> SELDPKGQHVCVASSPSAELQCCAGWRQKDQECTIPICEGPDACQKDEVCVKPGLCRCKPGFFGAHCSSRCPGQYWGPDCRESCPCHPHGQCEPATGACQCQADRWGARCEFPCACGPHGRCDPATGVCHCEPGWWSSTCRRPCQCNTAAARCEQATGACVCKPGWWGRRCSFRCNCHGSPCEQDSGRCACRPGWWGPECQQSRHHHHHH

SCARF1 (scavenger receptor class F member 1, SREC-1 or SR-F1) is a type I transmembrane protein that recognizes multiple endogenous and exogenous ligands such as modified low-density lipoproteins (LDLs) and is important for maintaining homeostasis and immunity. SCARF1 (MW, 86 kD) is a type I transmembrane protein that has a short signal peptide followed by a long extracellular region, a transmembrane helix, and a large cytoplasmic portion (Adachi et al., 1997). Its ectodomain has three glycosylation sites and contains multiple EGF-like domains, which usually has a two-stranded β-sheet followed by a loop region and three conserved disulfide bonds. Here, we solve the crystal structures of the N-terminal fragments of human SCARF1, which show that SCARF1 forms homodimers and its epidermal growth factor (EGF)-like domains adopt a long-curved conformation.

Among them, two fragments (f1, 20–132aa and f2, 20–221aa) were crystallized and the crystals diffracted to 2.2 Å and 2.6 Å, respectively. The structure of f2 fragment was solved by molecular replacement using the structure of f1 fragment combined with the EGF-like fragments predicted by AlphaFold as phasing models and refined to 2.6 Å resolution. The crystal belongs to space group P4122 with one molecule per asymmetric unit. In the f2 crystal structure, the N-terminal region of SCARF1 (residue 20–56aa) and the C-terminal region (210–221aa) are largely missing, suggesting these regions are quite flexible, consistent with low electron density of the N-terminal end of the f1 crystal. Rest of the f2 fragment adopts a long-curved conformation with multiple EGF-like domains arranged in tandem. Interestingly, in the crystal of f2 fragment, although an asymmetric unit has only one molecule, the dimer related by the crystallographic twofold symmetry can be well superimposed with the dimer found in the asymmetric unit of f1 crystals, suggesting that dimerization occurs in a similar fashion for the two fragments in different crystal forms. At the dimeric interfaces of f1 and f2 fragments, hydrogen bonds are formed between S88 and Y94 of the monomers, and F82 and Y94 are also close to each other, thus may form π-π interaction. But the salt bridges are not found in f2 crystals, suggesting they are not required for dimerization. To identify the binding site for modified LDLs on the region identified above (133–221aa), we calculated the surface electrostatic potential of the region based on the crystal structure of f2 fragment and found a positively charged area in this region, which is mainly composed of two sites, one is R160 and R161 (Site 1), the other is R188 and R189 (Site 2). The triple or quadruple mutants, R160S/R161S/R188S, R160S/R188S/R189S, and R160S/R161S/R188S/R189S, where positive charges are largely removed for the two sites, almost lost binding activities with modified LDLs completely, suggesting these arginines are crucial for lipoprotein interaction and both sites contribute to the recognition.1-[(2,4-dimethyl-1,3-thiazol-5-yl)methyl]-6-[[(1-methylcyclopropyl)amino]-bis(oxidanyl)-$l^{4}-sulfanyl]-3-[(1-methylpyrazol-4-yl)methyl]quinazoline-2,4-dione | C23 H28 N6 O4 S2 | 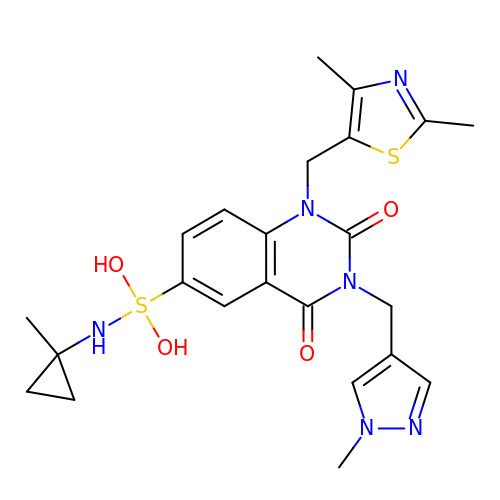IXVFSHGQJPQPKQ-UHFFFAOYSA-N>[2x]MSTSLLFEQLNFLILVAAEAELPIAHSTRKLLMDNSCNNCQIYELYNENLKDVKTDKDWFMNKFGPQTVHFVISNTINFPFYKIVYFDLLIPVVSHTWVQDSVKTKRHLRTNMYSPNPFHLLRDCQVYISKSSFNKCEYILYSDLLHLLGGTLVNYISNRTTHVIVQSPQDPIIATVSKLTFGSFSSSSTNKHTEKPLREWKFVYPIWILYHFKMAKPLKGELATLCELDMQDTSEEQLFAKWEEVIGDKQTSSSQLTLHPNKTLFKNHHFAISPDLNFFTPLYWFLKGFIEDLDGKVTPLSFSDDLKSVYQAFPDIDCYIGHSANSPILEKTKSIKPEIHVGNVSWLFYMFALQKFTPVSQCKLIHQPFHAKLFTSKELTVAYTNYFGSQRFYIQRLVEILGGLSTPELTRKNTHLITKSTIGKKFKVAKKWSLDPQNAIIVTNHMWLEQCYMNNSKLNPKDSRFQNFKLDDNMGWNIGQIGMDHSSLPTPKNLSMVTYD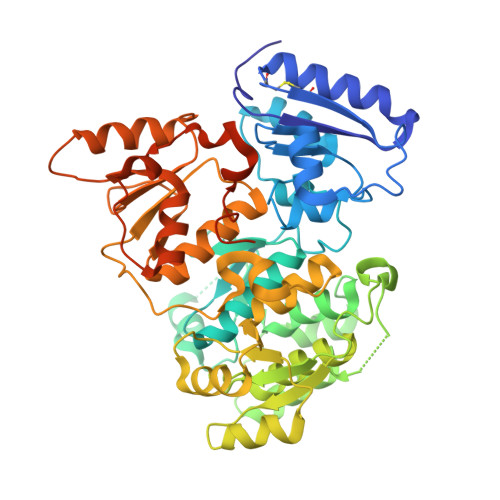TQSISEKPPPTN> A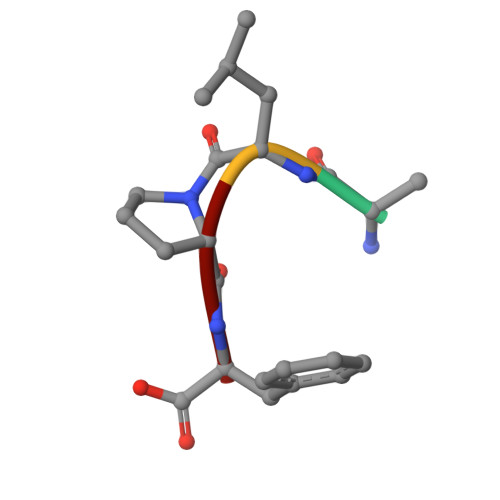LPF> MAKEWGYASHNGPDHWHELFPNAKGENQSPIELHTKDIRHDPSLQPWSVSYDGGSAKTILNNGHTCRVVFDDTYDRSMLRGGPLPGPYRLRQFHLHWGSSDDHGSEHTVDGVKYAAELHLVHWNPKYNTFKEALKQRDGIAV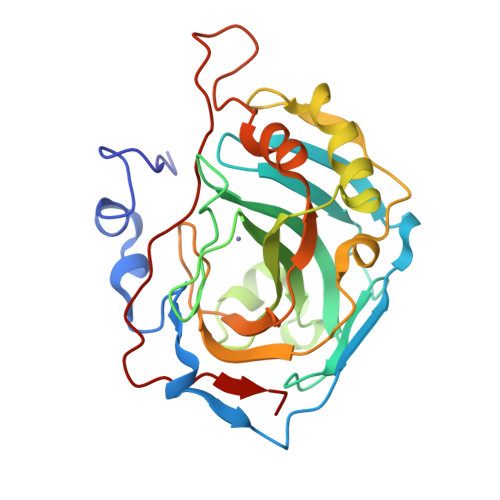IGIFLKIGHENGEFQIFLDALDKIKTKGKEAPFTKFDPSSLFPASRDYWTYQGSFTTPPCEECIVWLLLKEPMTVSSDQMAKLRSLLSSAENEPPVPLVSNWRPPQPINNRVVRASFK>[2x]MSVPTWNGFSLYTDETVRNAARYAYDNYLGKPYTGTVEATPVNFGGQMVYRQHHGLAHTLRTMAYAEIIVEEARKAKLRGESLKTFADGRTLADVTPEELRKIMIAQAFFVTGRDDEESSKNYEKYHEQSRDAFLKYVEENKSTLIPDVFKDEKDVKFYADVIEDKDHKWADSPAHVLVNQGHMVDLVRVKQPPESYLEYYFSQLQPWIGSTATEAVFATQRQFFHATYEAVAGFDSENKEPHLVVDGLGRYVIGQDGNPIREESDDEDEEESGELKFFSQKKKLEENQRYMRVDEYLKLDEVQKRFPGAGKKLDGGLPGLKEYQYLQRLNSINRARCENDVDFCLGQLQTAHHQTKITPIKRAFQSSSEKARRQPNMDEIAAARIVQQIMANPDCIHDDHVFLNGQKLEE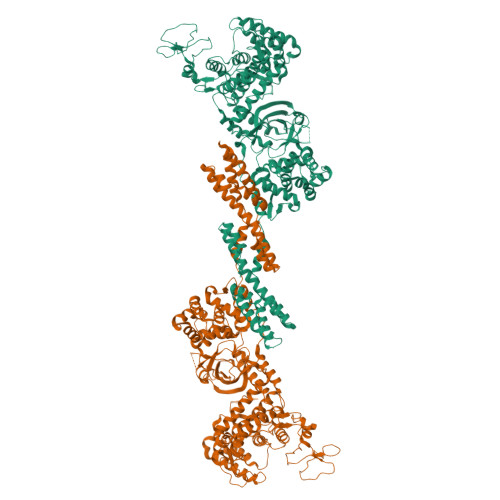KFFRDLLAKCDMAIVGSLLNDTDIRNIDTLMQHERNTEFHSTDAKAKPVKLGETWEKTIRSGGGVTQIKHDLIFLMQNDAWYHTRVNAIAQNRDKDSTFKEVLITALMTPLTNKSLMDTSRSPAPKTLFRGLDLSEEFKNKLINQAETIIANTTEHLFTDLSTEAFKQIKLNDFSQVSARTCASTSTNIEVPRTIFGSNTIFEILDPDGLLHPKQVGTHVSGSESEYSIYLPEDVALVPIKVSFDGKTGKGKDRHIFTLVAVKSPDFTPRHESGYAVGPLLKMQTPKLEEIQRLVEQAREEPDLERVFNLQSRVARQAKFSTESGYKTFLNEKVAPVLEQSLNGLLDNNVTILGKVLSAFPSDGQWSAFNSVEARQMKIQMDAIKQMVEKKAVLEGQILPALAQCQNALEKQNIAGALQALRNIPSLEHHHHHH4,4-dimethyl-1,2,3,4-tetrahydroisoquinoline 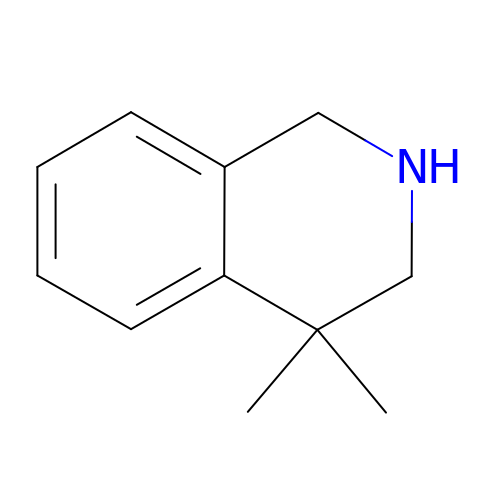| C11 H15 N | QOWZBQAJZICMKD-UHFFFAOYSA-N methyl (~{Z})-3-(4-hydroxyphenyl)-2-methyl-prop-2-enoate | C11 H12 O3 | 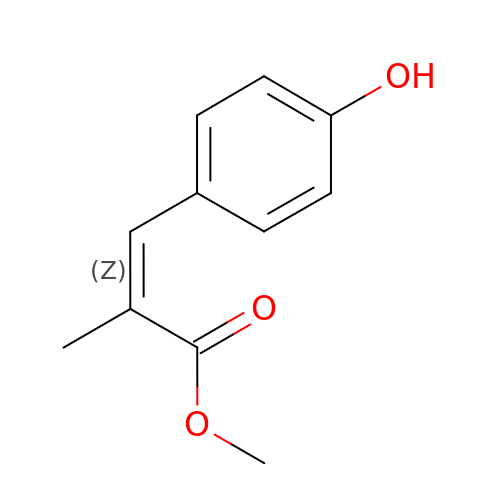CPKCCIUDOPJZSI-FPLPWBNLSA-N>[4x]MPYPKKVTIKEVGPRDGLQNEPVWIATEDKITWINQLSRTGLSYIEITSFVHPKWIPALRDAIDVAKGIDREKGVTYAALVPNQRGLENALEGGINEACVFMSA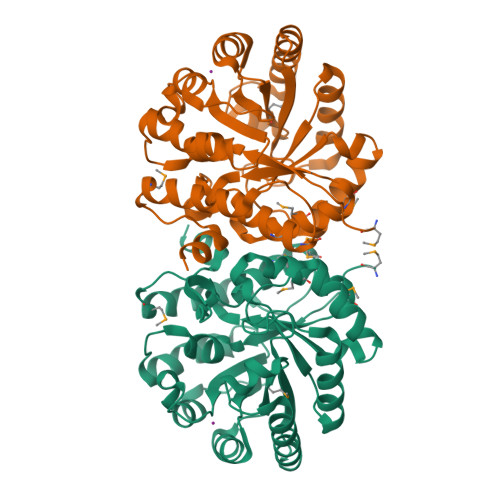SETHNRKNINKSTSESLHILKQVNNDAQKANLTTRAYLSTVFGCPYEKDVPIEQVIRLSEALFEFGISELSLGDTIGAANPAQVETVLEALLARFPANQIALHFHDTRGTALANMVTALQMGITVFDGSAGGLGGCPYAPGSSGNAATEDIVYMLEQMDIKTNVKLEKLLSAAKWIEEKMGKPLPSRNLQVFKSSLEHHHHHH> 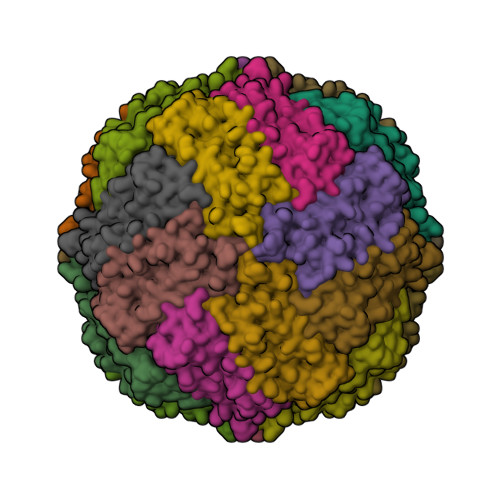MSSQIRQNYSTDVEAAVNSLVNLYLQASYTYLSLGFYFDRDDVALEGVSHFFRELAEEKREGYERLLKMQNQRGGRALFQDIKKPAEDEWGKTPDAMKAAMALEKKLNQALLDLHALGSARTDPHLCDFLETHFLDEEVKLIKKMGDHLTNLHRLGGPEAGLGEYLFERLTLKHD>[2x]GAMAPPRKVLIISAGASHSVALLSGDIVCSWGRGEDGQLGHGDAEDRPSPTQLSALDGHQIVSVTCGADHTVAYSQSGMEVYSWGWGN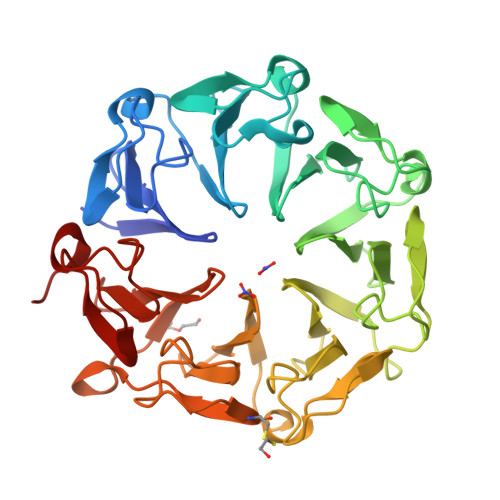FGRLGHGNSSNLFTPLPIKALHGIRIKQIACGDSHCLAVTMEGEVQSWGRNQNGQLGLGDTEDSLVPQKIQAFEGIRIKMVAAGAEHTAAVTEDGDLYGWGWGRYGNLGLGDRTDRLVPERVTSTGGEKMSMVACGWRHTISVSYSGALYTYGWSKYGQLGHGDLEDHLIPHKLEALSNSFISQISGGARHTMALTSDGKLYGWGWNKFGQVGVGNNLDQCSPVQVRFPDDQKVVQVSCGWRHTLAVTERNNVFAWGRGTNGQLGIGESVDRNFPKIIEALSVDG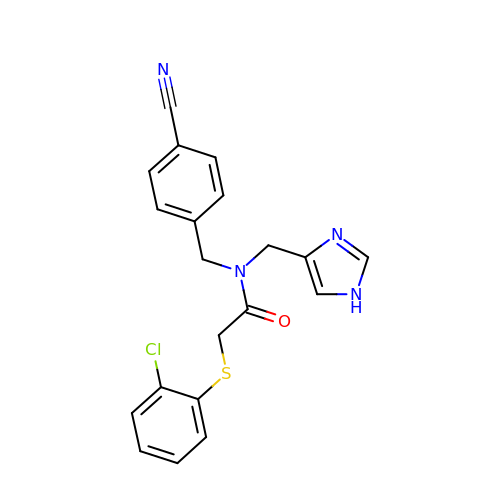2-(2-chlorophenyl)sulfanyl-~{N}-[(4-cyanophenyl)methyl]-~{N}-(1~{H}-imidazol-4-ylmethyl)ethanamide | C20 H17 Cl N4 O S | LSTBXSJHAMGXJT-UHFFFAOYSA-N>[2x]TKTGYINAAFRSSRNNEAYLFINDKYVLLDYAPGTSNDKVLYGPSFVRDGYKSLAKTIFGTYGIDCSFDTEYNEAFIFYENFCARIDYAPHSDKDKIISGPKKIADMFPFFKGTVFEN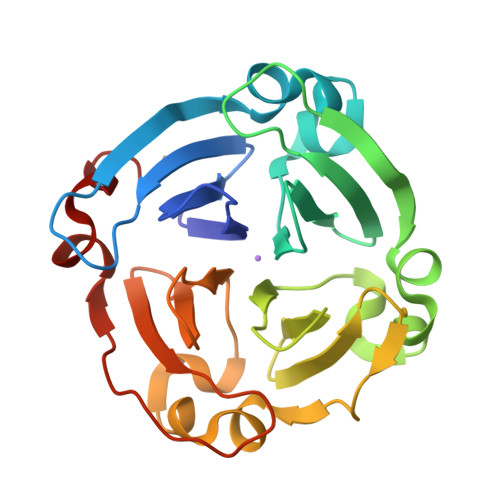GIDAAFRSTKGKEVYLFKGDKYARIDYLTNRLVQNIKSISDGFPCLRGTIFEAGMDSAFASHKTNEAYLFKGEYYARINFTPGSTNDIMGGVKKTLDYWPSLRGIIPLE> AKKNLPTAPP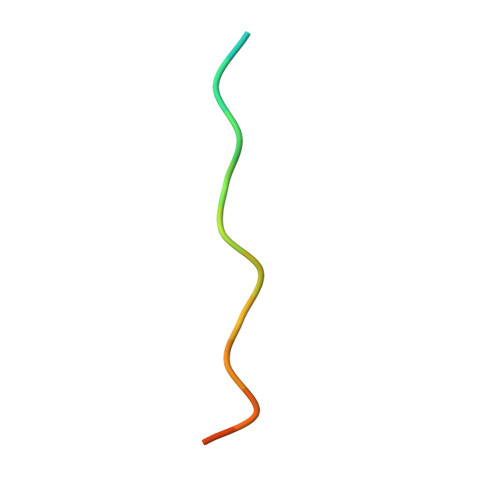RRRVSE> MSVTVKRIIDNTVIVPKLPANEDPVEYPADYFRKSKEIPLYINTTKSLSDLRGYVYQGLKSGNVSIIHVNSYLYGALKDIRGKLDKDWSSFGINIGKAGDTIGIFDLVSLKALDGVLPDGVSDASRTSADDKWLPLYLLGLYRVGRTQMPEYRKKLMDGLTNQCKMINEQFEPLVPEGRDIFDVWGNDSNYTKIVAAVDMFFHMFKKHECASFRYGTIVSRFKDCAALATFGHLCKITGMSTEDVTTWILNREVADEMVQMMLPGQEIDKADSYMPYLIDFGLSSKSPYSSVKNPAFHFWGQLTALLLRSTRARNARQPDDIEYTSLTTAGLLYAYAVGSSADLAQQFCVGDNKYTPDDSTGGLTTNAPPQGRDVVEWLGWFEDQNRKPTPDMMQYAKRAVMSLQGLREKTIGKYAKSEFDK;>[2x]MSSLKKILGLKGKGKKSKKLGIAPPPYEEDTSMEYAPSAPIDKSYFGVDEMDTYDPNQLRYEKFFFTVKMTVRSNRPFRTYSDVAAAVSHWDHMYIGMAGKRPFYKILAFLGSSNLKATPAVLADQGQPEYHAHCEGRAYLPHRMGKTPPMLNVPEHFRRPFNIGLYKGTIELTMTIYDDESLEAAPMIWDHFNSSKFSDFREKALMFGLIVEKKASGAWVLDSISHFK

Vesicular stomatitis virus (VSV) is a negative-strand RNA virus with a non-segmented genome, closely related to rabies virus. The VSV RNP complex assembles, together with M, into a helical, bullet-shaped structure, as it buds through the plasma membrane of an infected cell. The asymmetric unit of the VSV helical nucleocapsid, which repeats every 9 RNA nucleotides, contains one nucleoprotein (N) subunit and two (chemically identical) matrix protein subunits (M1 and M2). N is an elongated, two-lobed protein of ~420 amino-acid residues; the single stranded RNA binds in a cleft between the two lobes, with nine nucleotides per N subunit.

We obtained a helical reconstruction of the trunk at 4.1 Å resolution, and a local reconstruction of the basic building module (one N and two M proteins) at 3.5 Å resolution. Helical reconstructions calculated from segments that belonged to unflattened classes showed substantially improved resolution, the best being the reconstruction obtained from the 38.5 subunits-per-turn class, which had an overall resolution of 4.1 Å as judged by Fourier shell correlation (FSC) analysis. The model from the local reconstruction map was then also placed into the N = 38.5 helical reconstruction and refined at 4.1 Å resolution and rigid-body fitted into the maps for the other N classes. The innermost layer is the RNA-N protein (RNP) complex, which coils into a left-handed helix with a polarity such that the 3′ end of the (-)-strand genomic RNA is at the tip of the bullet-shaped virions and the 5′ end at the blunt end of the trunk. Two layers of matrix protein (M) surround the RNP, with the same helical symmetry, but with a different packing within each layer. A local resolution estimate for the N = 38.5 helical reconstruction and analysis of the refined temperature factors in our model show that the outer matrix protein (M2) layer is less well defined than the inner matrix protein (M1) layer. We explain this observation by partial occupancy of M2-layer subunits in the outer layer, consistent with the reported stoichiometry of only 1.5 M proteins per N protein in virions. As evident from the superposition of two adjacent asymmetric units on a single common nucleoprotein subunit, the molecular contacts that govern coiling of the RNP ribbon into a helix are not fundamentally altered when the number of subunits per helical turn changes from 34.5 to 41.5 between different virions. To describe the subunit interactions within the helical nucleocapsid, we classified the interfaces according to whether they are within a layer (lateral and axial intra-layer contacts for the N, M1, and M2 layers) or between layers (radial inter-layer contacts). Table 1 summarizes the observed interfaces in the N = 38.5 helical structure together with the calculated interface areas (IA), or buried accessible surface areas, for each of the contacts.> SEMASEIHMTGPMCLIENTNGRLMANPEALKILSAITQPMVVVAIVGLYRTGKSYLMNKLAGKKKGFSLGSTVQSHTKGIWMWCVPHPKKPGHILVLLDTEGLGDVEKGDNQNDSWIFALAVLLSSTFVYNSIGTINQQAMDQLYYVTELTHRIRSKSSPDENENEVEDSADFVSFFPDFVWTLRDFSLDLEADGQPLTPDEYLTYSLKLKKGTSQKDETFNLPRLCIRKFFPKKKCFVFDRPVHRRKLAQLEKLQDEELDPEFVQQVADFCSYIFSNSKTKTLSGGIQVNGPRLESLVLTYVNAISSGDLPCMENAVLALAQIENSAAVQKAIAHYEQQMGQKVQLPTETLQELLDLHRDSEREAIEVFIRSSFKDVDHLFQKELAAQLEKKRDDFCKQNQEASSDRCSALLQVIFSPLEEEVKAGIYSKPGGYRLFVQKLQDLKKKYYEEPRKGIQAEEILQTYLKS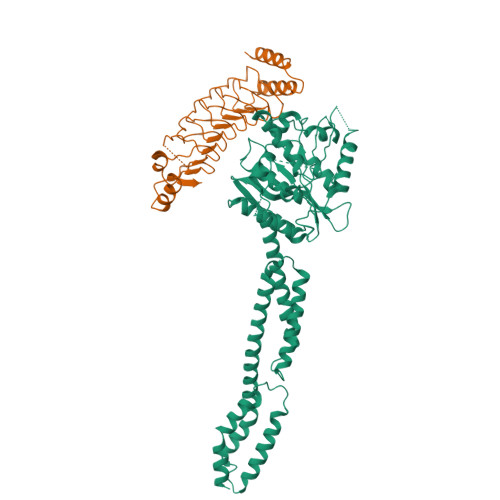KESMTDAILQTD;> SGRPMTYADYFSAWDKWEKQALPGEERDEAVSRLKECLINNSDELRLDRLNLSSLPDNLPAQITLLNVSYNQLTNLPELPVTLKKLYSASNKLSELPVLPPALESLQVQHNELENLPALPDSLLTMNISYNEIVSLPSLPQALKNLRATRNFLTELPAFSEGNNPVVREYFFDRNQISHIPESILNLRNECSIHISDNPLSSHALPALQRLTSSPDYHGPRIYFSMSDGQQNTLHR> MNDDRETPPKRKPGEDDTLFDIDFLDDTTSHSGSRSKVTNSHANANYIPPSHVLPEETIDLDADDDNIENDVHENLFMSNNHDDQTSWNANRFDSDAYQPQSLRAVKPPGLFARFGNGLKNAFTFKRKKGPESFEMNHYNAVTNNELDDNYLDSRNKFNIKILFNRYILRKNVGDAEGNGEPRVIHINDSLANSSFGYSDNHISTTKYNFATFLPKFLFQEFSKYANLFFLCTSAIQQVPHVSPTNRYTTIGTLLVVLIVSAMKECIEDIKRANSDKELNNSTAEIFSEAHDDFVEKRWIDIRVGDIIRVKSEEPIPADTIILSSSEPEGLCYIETANLDGETNLKIKQSRVETAKFIDVKTLKNMNGKVVSEQPNSSLYTYEGTMTLNDRQIPLSPDQMILRGATLRNTAWIFGLVIFTGHETKLLRNATATPIKRTAVEKIINRQIIALFTVLIVLILISSIGNVIMSTADAKHLSYLYLEGTNKAGLFFKDFLTFWILFSNLVPISLFVTVELIKYYQAFMIGSDLDLYYEKTDTPTVVRTSSLVEELGQIEYIFSDKTGTLTRNIMEFKSCSIAGHCYIDKIPEDKTATVEDGIEVGYRKFDDLKKKLNDPSDEDSPIINDFLTLLATCHTVIPEFQSDGSIKYQAASPDEGALVQGGADLGYKFIIRKPNSVTVLLEETGEEKEYQLLNICEFNSTRKRMSAIFRFPDGSIKLFCKGADTVILERLDDEANQYVEATMRHLEDYASEGLRTLCLAMRDISEGEYEEWNSIYNEAATTLDNRAEKLDEAANLIEKNLILIGATAIEDKLQDGVPETIHTLQEAGIKIWVLTGDRQETAINIGMSCRLLSEDMNLLIINEETRDDTERNLLEKINALNEHQLSTHDMNTLALVIDGKSLGFALEPELEDYLLTVAKLCKAVICCRVSPLQKALVVKMVKRKSSSLLLAIGDGANDVSMIQAAHVGVGISGMEGMQAARSADIAVGQFKFLKKLLLVHGSWSYQRISVAILYSFYKNTALYMTQFWYVFANAFSGQSIMESWTMSFYNLFFTVWPPFVIGVFDQFVSSRLLERYPQLYKLGQKGQFFSVYIFWGWIINGFFHSAIVFIGTILIYRYGFALNMHGELADHWSWGVTVYTTSVIIVLGKAALVTNQWTKFTLIAIPGSLLFWLIFFPIYASIFPHANISREYYGVVKHTYGSGVFWLTLIVLPIFALVRDFLWKYYKRMYEPETYHVIQEMQKYNISLVPRGSDSRPHVQQFQNAIRKVRQVQRMKKQRGFAFSQAEEGGQEKIVRMYDTTQKRGKYGELQDASANPFNDNNGLGSNDFESAEPFIENPFADGNQNSN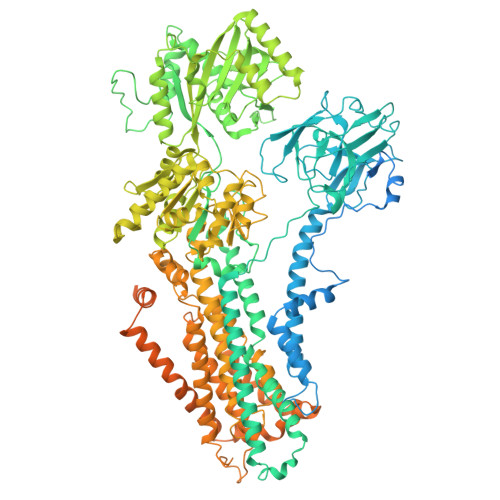RFSSSRDDISFDIGGGGLVPRGSGGTAAAPGPAPAPAPASAPAAAAPAGAGTPVTAPLAGTIWKVLASEGQTVAAGEVLLILEAMKMETEIRAAQAGTVRGIAVKAGDAVAVGDTLM>STAGKVIKCKAAVLWEEKKPFSIEEVEVAPPKAHEVRIKMVATGICRSDDQVVSGTLVTPLPVIAGHEAAGIVESIGEGVTTVRPGDKVIPLFTPQCGKCRVCKHPEGNFCLKNDLSMPRGTMQDGTSRFTCRGKPIHHFLGTSTFSQYTVVDEISVAKIDAASPLEKVCLIGCGFSTGYGSAVKVAKVTQGSTCAVFGLGGVGLSVIMGCKAAGAARIIGVDINKDKFAKAKEVGATECVNPQDYKKPIQEVLTEMSNGGVDFSFEVIGRLDTMVTALSCCQEAYGVSVIVGVPPDSQNLSMNPMLLLSGRTWKGAIFGGFKSKDSVPKLVADFMAKKFALDPLITHVLPFEKINEGFDLLRSGESIRTI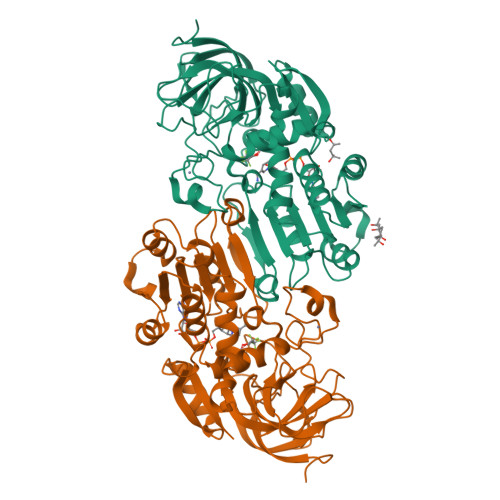LTF[2x]> MASVHGTTYELLRRQGIDTVFGNPGSNELPFLKDFPEDFRYILALQEACVVGIADGYAQASRKPAFINLHSAAGTGNAMGALSNAWNSHSPLIVTAGQQTRAMIGVEALLTNVDAANLPRPLVKWSYEPASAAEVPHAMSRAIHMASMAPQGPVYLSVPYDDWDKDADPQSHHLFDRHVS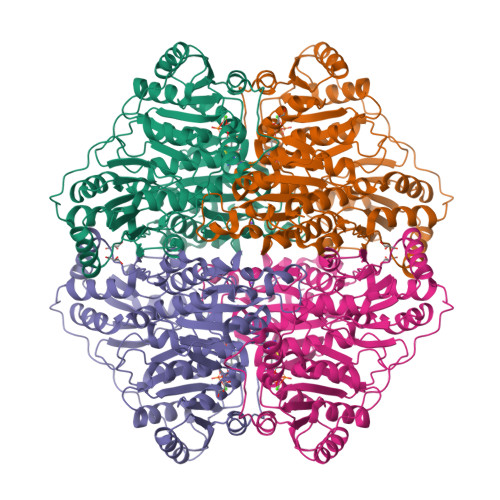SSVRLNDQDLDILVKALNSASNPAIVLGPDVDAANANADCVMLAERLKAPVWVAPSAPRCPFPTRHPCFRGLMPAGIAAISQLLEGHDVVLVIGAPVFRYHQYDPGQYLKPGTRLISVTCDPLEAARAPMGDAIVADIGAMASALANLVEESSRQLPTAAPEPAKVDQDAGRLHPETVFDTLNDMAPENAIYLNESLSTTAQMWQRLNMRNPGSYYFCAAGGLGFALPAAIGVQLAEPERQVIAVIGDGSANYSISALWTAAQYNIPTIFVIMNNGTYGYLRWFAGVLEAENVPGLDVPGIDFRALAKGYGVQALKADNLEQLKGSLQEALSAKGPVLIEVSTVSPVKRSHHHHHH>[2x]GHVAPAPAPAPEVQTKHFTLKSDVLFNFNKSTLKPEGQQALDQLYSQLSNL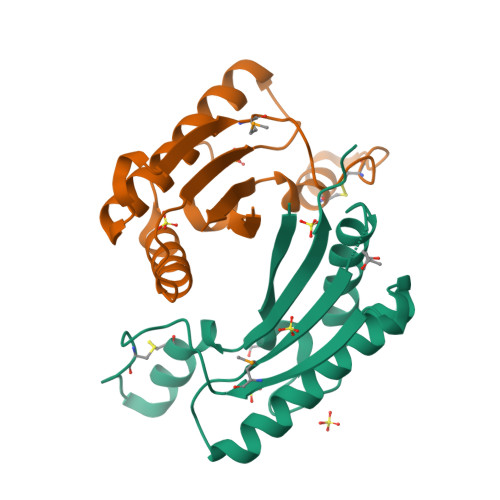DPKDGSVVVLGFTDRIGSDAYNQGLSEKRAQSVVDYLISKGIPSDKISARGMGESNPVTGNTCDNVKPRAALIDCLAPDRRVEIEVKGVKDVVGS>GQDMVSPPPPIADEPLTVNTGIYLIECYSLDDKAETFKVNAFLSLSWKDRRLAFDPVRSGVRVKTYEPEAIWIPEIRFVNVENARDANVVDISVSPDGTVQYLERFSARVLSPLDFRRYPFDSQTLHIYLIVRSVDTRNIVLAVDLEKVGKNDDVFLTGWDIESFTAVVKPANFALEDRLESKLDYQLRISRQYFSYIPNIILPMLFILFISWTAFWSTSYEANVTLVVSTLIAHIAFNILVETNLPKTPYMTYTGAIIFMIYLFYFVAVIEVTVQHYLKVESQPARAASITRASRIAFPVVFLLANIILAFLFFGF[5x]

At present, the best structurally characterized pLGIC is the G. violaceus ligand-gated ion channel (GLIC), of prokaryotic origin. Each subunit consists of an extracellular domain (ECD), predominantly in a β-sandwich fold, and a transmembrane domain (TMD) composed of four helices, labeled M1–M4. However, the GLIC is a pH-gated channel, activated by lowering the pH, with a maximal activation at pH 4 and a pH50 around 5. We instead found that proton activation is a complex multiple loci mechanism, with the key contribution stemming from the coupling interface between the extracellular and transmembrane domain, with E35 acting as a key proton-sensing residue.

The mutant of the vestibular pair on the β5 strand, D86N-D88N, yields a significant decrease in pH50 greater than 1 pH unit. All residues were also tested individually, with most mutations having no significant effect, although a large majority tend to decrease the pH50 (notably D86N/A, D88N/A, and D91N). Mutation of Asp/Glu residues at the complementary (−) face, in general, decreased the proton sensitivity of the GLIC, with additive effects in many cases, especially for D88 and D86. However, the pattern of phenotypes does not allow discriminating whether those residues are involved in proton sensing or gating, because mutations to Asn/Gln also produced decreased proton sensitivity. A structural analysis was performed on E26Q, E26A, E35Q, E35A, E67A, E75A, E82Q, E82A, D86A, D88N, D88A, H127N, E181A, and H277Q mutants, by solving their structure at pH 4. The key mutants at E26, D86, and D88 were solved at pH 4, each showing a structure similar to that of the Wt. All structures were in the apparently open conformation.> KGQEGSVCLRSSDCASGLCCARHFWSKICKPVLKEGQVCTKHRRKGSHGLEIFQRCYCGEGLSCRIQKDHHQASNSSR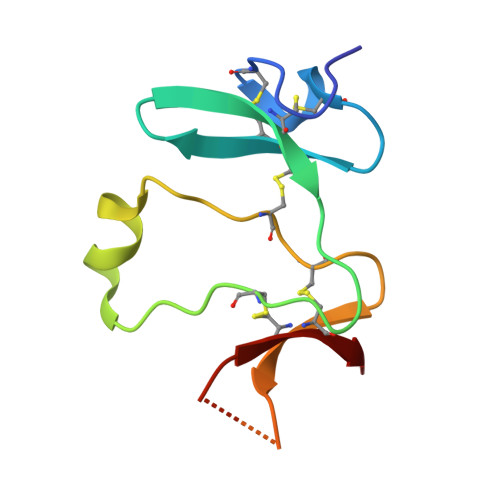LHTCQRH>[2x]PMILGYWNVRGLVHPIRLLLEYTDSSYEEKRYAMGDAPDYDRSQWLNEKFKLGLDFPNLPYLIDGSRKITQSNAIMRYLARKHHLCGE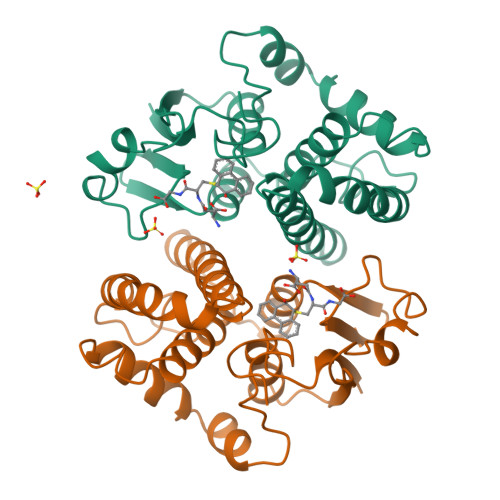TEEERIRADIVENQVMDNRMQLIMLCYNPDFEKQKPEFLKTIPEKMKLYSEFLGKRPWFAGDKVTYVDFLAYDILDQYHIFEPKCLDAFPNLKDFLARFEGLKKISAYMKSSRYLSTPIFSKLAQWSNK> GSMTEIALIGNPNSGKTSLFNLITGHNQRVGNWPGVAVERKSGLVKKNKDLEIQDLPGIYSMSPYSPEEKVARDYLLSQRADSIL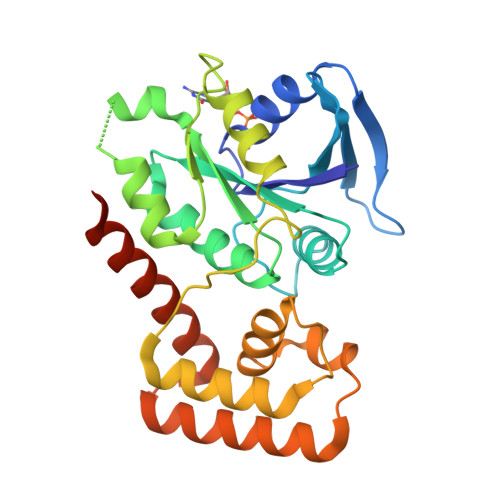NVVDATNLERNLYLTTQLIETGIPVTIALNMIDVLDGQGKKINVDKLSYHLGVPVVATSALKQTGVDQVVKKAAHTTTSTVGDLAFPIYDDRLEAAISQILEVLGNSVPQRSARFYAIKLFEQDSLVEAELDLSQFQRKEIEDIIRITEEIFTEDAESIVINERYAFIERVCQMAESHTEDFALTLS Biuret hydrolase (BiuH) hydrolyzes biuret to allophanate and is part of the Isochorismatase-like hydrolase (IHL) protein family within the cysteine hydrolase superfamily. TrtA is a member of the isochorismatase-like hydrolase (IHL) protein family, similarly to BiuH, and has a catalytic efficiency (kcat/KM) of 6 x 105 M−1s−1, a KM for triuret of 20 μM, and exquisite substrate specificity. TrtA and BiuH are members of the IHL protein family that possess the catalytic triad comprised of a cysteine, aspartate, and lysine residue. Interestingly, the active sites of TrtA and BiuH are almost identical in sequence, and so it was hypothesized that triuret is the substrate for TrtA, funneling into biuret metabolism.

However, the inactive mutant C162S was able to produce large cocrystals with biuret. The cocrystal containing biuret, at a concentration of 30 mM biuret, only occupied one of four active sites in the unit cell. Biuret is coordinated by a subset of the residues that coordinate triuret, and it binds in a noncatalytic fashion. The dihedral angle for biuret is fairly planar in this structure and binds in the same place where triuret is planar as well. The closed conformation is observed in all of the chains of the triuret cocrystal as well as for a single chain in the biuret cocrystal, which has biuret bound. The other chains in the biuret cocrystal that do not have biuret bound, as well as the apo WT crystal, are in the open conformation. Biuret shows very low activity and is a very weak inhibitor of TrtA. Inhibition data suggests that biuret is a competitive inhibitor. The biuret cocrystallized with TrtA binding in a noncatalytic fashion suggesting that the glutamine residue has a strong role in binding the substrate and stabilizing the preattack conformation as biuret is fairly planar in this structure.

>[4x]GSHMIRIDATPYPYQFHPRSTALVVIDMQRDFIEEGGFGSALGNDVRPLAAIVPTVAALLQLAREAGMLVVHTRESHLPDLSDCPRSKRLRGNPTLGIGDVGPMGRILVQGEPGNQILPQLAPVEGELVIDKPGKGAFYATDLHAQLQERRITHLLVAGVTTEVSVQTSMREANDRGYECLVIEDACASYFPDFHRITLEMLTAQGGIVGWRTPLAQLQAGVA> FVGGFHTRSESSLENFLGRA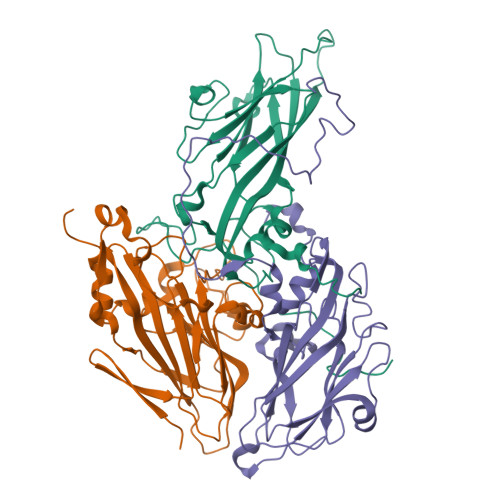ANTYRTSFKTLSTKPSLKFASWTITTRKVAMLRRKMEMFTYMRFDVEVTFVITSSKCKSDPSSGSLPVLTFMVQYVPPGGPVPSSVDSFSWQSSTNPSIFWTQGNAPPRMSIPYMSIGNAYSNYYDGYSHHGADGVYGYNTLNNQGQLYFRHVNSSNPGAYTCVVKIYFKLQHVKAWVPRPPRLCNYQRAENVNFKVQGVTDTKESITANPG;> SSNVRSITLGNSTITTQESSNVVVGFGVWPSYLSKSKSGSGSTQPTQPDTATERFYTLESVKWQKTDNGWYWKFPDALKDMGLFGQNMLYHFLGRTGWTIHVKCEASRFFQGALLVVCVPQAEKGCAVITRDVNATALDEGDKAKKFTAGSVSSQNGVQTAVYNAAMGVAVGNLTIFPHQWINLKTNNSATIVKPYINSIPMENMYRHFNFTLMVIPFVPLEWSVGACTYVPITVTVAPQNAEYIGLRLA;> GNPTQLVPGSNMYLTSDDFRSPEAMPQFEVTPEMFIPGEVHNLMEIAETDSTVPVNNVGMAVNSMEAYRIGVNPNTGSGTQVYGWPLNPGKSSVFKRTNLGEILNYFAHWSGSIQLTFVFCGSAQATGKFLLAYSPPGAGAPTDRKGARLGTHVVWDVGLQSSCVLEVPWISNTFYRKDKSSGTGFSKAGYVTCWFQTSIVAPADAMSKCYIMCFVSADNDFSVRLLKDTPFIKEQAARRV> GIQGLAKLIADVAPSAIRENDIKSYFGRKVAIDASMSIYQFLIAVRQGGDVLQNEEGETTSHLMGMFYRTIRMMENGIKPVYVFDGKPPQLKSGELAKRSERRAEAEKQLQQAQAAGAEQEVEKFTKRLVKVTKQHNDECKHLLSLMGIPYLDAPSEAEASCAALVKAGKVYAAATEDMDCLTFGSPVLM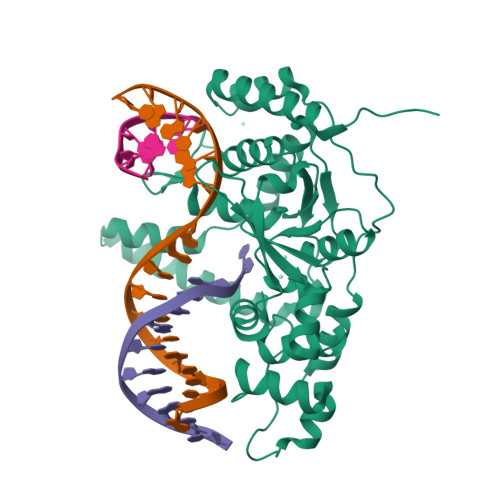RHLTASEAKKLPIQEFHLSRILQELGLNQEQFVDLCILLGSDYCESIRGIGPKRAVDLIQKHKSIEEIVRRLDPNKYPVPENWLHKEAHQLFLEPEVLDPESVELKWSEPNEEELIKFMCGEKQFSEERIRSGVKRLSKSRQGSTLEVLFQ> MSESELKVNQAVAAASDDNV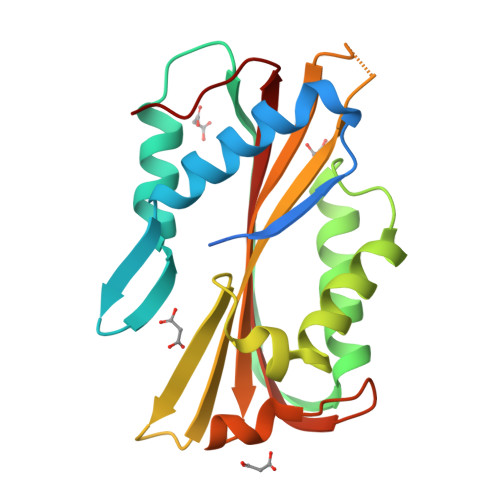FQPVDQLPEDLIPSSIQVLKFSGKYLKLEQNKAYFDWPEFKTAIDNYTGEDLSFDKYDQSTINQREQEVGSMVDKIAKFLRDAFSAVVDLSKLGAIILNTFTNLEEESSSGFLQFSTNNVKKNSSWEYRVLFSVPFGDNAPSYFYSLVTTILITADIEEKTGWWGLTSSTKKNFAVQIDALELVVKKGFKAPN>[6x]MSKTR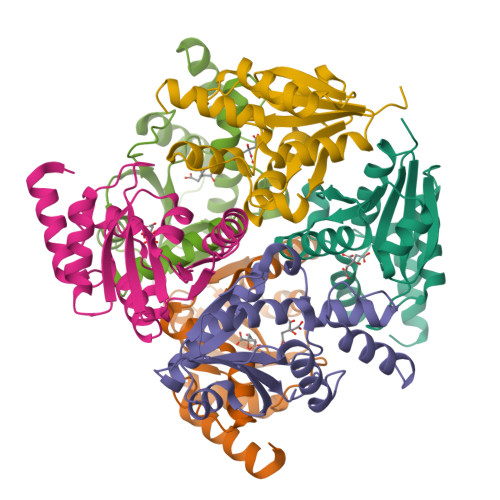VIYPGTFDPITNGHVDLVTRASRMFDEVVVAIAIGHHKNPLFSLEERVALAQSSLGHLSNVEFVGFDGLLVNFFKEQKATAVLRGLRAVSDFEYEFQLANMNRQLDPHFEAVFLTPSEQYSFISSTLIREIARLKGDVTKFVPQAVVEAFERKHQQGW>MIHEVDEVLKALLKGGALTDSGIDVAFEAPTRDWAARRNAPVVNAYLYDIREDVGRRHRGQVAVRDQDDIVVKRRQPPRWFRLSYLVTAWTKTPQDEHRLLSAVLATLLPREQLPPYELPGALGAMNLPVPMTVAGVQTESRSLAEIWSALGGELKPSLDLVVTAPFPAYPEYDAGPPVTEGATVRIGGVEGDPPMSEGRSHRPHQVAAARAARKAVTDGRTKRQ[6x];>[6x]MSLPKPEDVLVAPNFGIQIDGVMVEYLNSVSNLQIEQDVIRYQQNQGTTGRNNVTLMPGVAKDGSVQVERGMSQSSVFTQWINDSMAGRMATARKNATIIVMDYEDNPVKRWNLRNAWCSKVVAGTLKAGDTNALTETITIVFEELVVE;>MPSYLSPGVYVEEVASGSRPIEGVGIEGVGTSVAAFVGLAPTGPLNEPTLVTNWTQYVAAFGDFTGGYYLAHSVYGFFNNGGSAAYVVRVGGSAEDAAADGSVNGAAAPAAVTGSTAKALPAAEPKQLGTFAVTATAAGQSGPLTVEVADPEGEGPAERFKLIVKDGDKPVETFDVSAKKGNRSYVVTQVKERSKLITVTEAAPSAQLV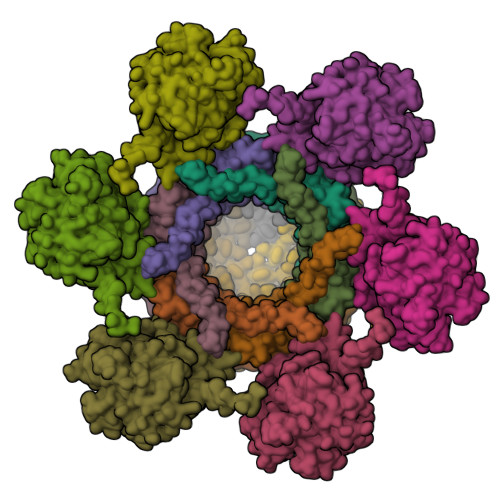RPENQSLTLPAPPSAAPAVPAGQAESAHPGPAQYLGDSSDRTGFGGLEAIDEISMVAVPDLMAAYQRGAIDLEAVKAVQLGLIAHCELMGDRVAIIDPPPNQNARQIRVWRQETAGYDSKYAALYYPWIKSFDPATGQSRLVPPSGHVAGIWARNDSERGVHKAPANEVVRGAVDLELQITRGEQDLLNPIGVNCIRSFPGRGIRVWGARTLSSDPAWRYLNIRRYFNYLEESILIGTQWVVFEPNDHNLWARIRRNVSAFLVNEWRNGALFGQSPDQAYYVKCDEETNPPESVDLGRVVCEIGIAPVKPAEFVIFRLAQFSSGGGELDE[6x]> MYDLLVIGAGPGGYVAAIRAAQLGMKVGVVEKEKALGGTCLRVGCIPSKALLETTERIYEAKKGLLGAKVKGVELDLPALMAHKDKVVQANTQGVEFLFKKNGIARHQGTARFLSERKVLVEETGEELEARYILIATGSAPLIPPWAQVDYERVVTSTEALSFPEVPKRLIVVGGGVIGLELGVVWHRLGAEVIVLEYMDRILPTMDLEVSRA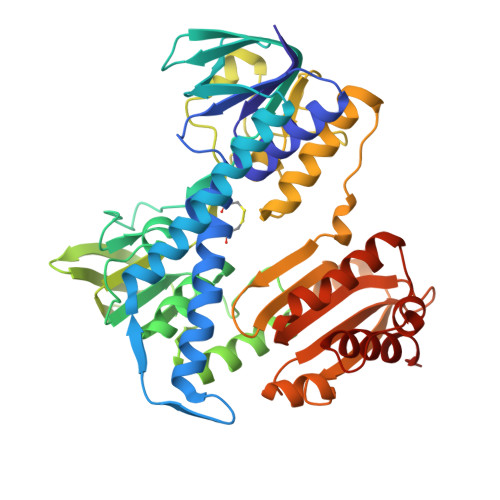AERVFKKQGLTIRTGVRVTAVVPEAKGARVELEGGEVLEADRVLVAVGRRPYTEGLSLENAGLSTDERGRIPVDEHLRTRVPHIYAIGDVVRGPMLAHKASEEGIAAVEHMVRGFGHVDYQAIPSVVYTHPEIAAVGYTEEELKAQGIPYKVGKFPYSASGRARAMGETEGFIKVLAHAKTDRILGVHGIGARVGDVLAEAALALFFKASAEDLGRAPHAHPSLSEILKEAALAAWERPIHL>MTNDNSGIWVLGYGSLIYKPPSHYTHRIPAIIHGFARRFWQSSTDHRGTPANPGRVATLIPYEDIIRQTAFLKNVNLYSESAPIQDPDDLVTIGVVYYIPPEHAQEVREYLNVREQNGYTLHEVEVHLETNREHEAELGEALEQLPRHNKSGKRVLLTSVYIGTIDNE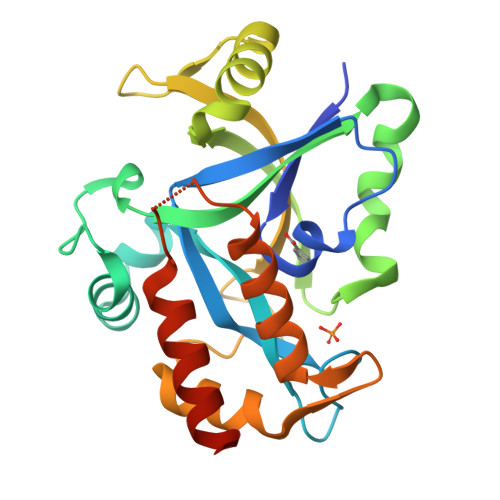AFVGPETVDETAKVIAVSHGPSGSNYEYLAKLEQALAQMPIMKERGRITDHYLTALLETVNKYRHHHHHHHH[2x]>[4x]QGAITLLTLIKTAEHWARQDIRTIEDSKLRALLTLCAVMTRKFSKSQLSLLCETHLRREGLGQDQAEPVLEVYQRLHSDKGG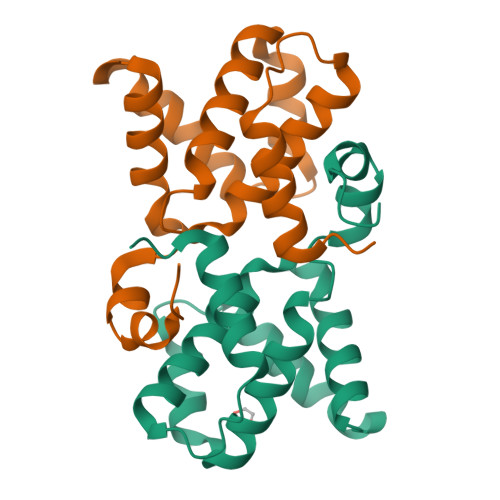SFEAALWQQWDRQSLIMFITAFLNIALQLPCESSAVVVSGLRTLVPQSDNEE> UGAGC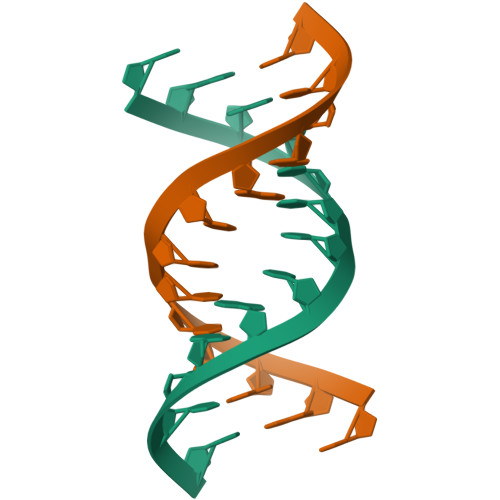UUCGGCUC>MTKIALIGSGQIGAIVGELCLLENLGDLILYDVVPGIPQGKALDLKHFSTILGVNRNILGTNQIEDIKDADIIVITAGVQRKEGMTREDLIGVNGKIMKSVAESVKLHCSKAFVICVSNPLDIMVNVFHKFSNLPHEKICGMAGILDTSRYCSLIADKLKVSAEDVNAVILGGHGDLMVPLQRYTSVNGVPLSEFVKKNMISQNEIQEIIQKTRNMGAEIIKLAKASAAFAPAAAITKMIKSYLYNENNLFTCAVYLNGHYNCSNLFVGSTAKINNKGAHPVEFPLTKEEQDLYTESIASVQSNTQKAFDLIKGHHHHHH[16x]

Malate dehydrogenase (PfMDH, EC 1.1.1.37) is located downstream of PfAspAT in the cytosol of the parasite. It catalyzes the reversible reaction from malate to oxaloacetate using the reduction of NAD+ to NADH, thus aiding in the maintenance of the correct redox environment, crucial for the parasite’s survival particularly during the blood stages. PfMDH is also involved in the shuttle mechanism of the TCA cycle intermediates (malate/oxaloacetate), necessary for electron transfer from cytosolic NADH to the mitochondrial electron transport chain, a validated antimalarial drug target. PfMDH is a globular tetrameric protein, where each monomer is comprised of 326 residues, which form 9 alpha helixes and 11 beta-sheets.

PfMDH-WT crystals belonged to P1 space group and diffracted to 2.4 Å. Molecular replacement yielded a clear solution of 4 tetramers in the asymmetric unit with R/Rfree of 0,25/0,26, respectively. Similarly to other NAD-dependent dehydrogenases, the active sites are located in the cleft between two domains: an N-terminal cofactor-binding domain containing a parallel structure of first six beta-sheets (Rossmann-fold) and C-terminal substrate-binding domain. The oligomeric surfaces of PfMDH can be split into two major groups: AB and AC. These surfaces comprise 1852.9 Å2 (AB) and 1372.1 Å2 (AC), respectively. Active sites from subunits A and B mirror each other and are located in close proximity to the AB interface (but well separated from each other and interface residues) and distal to the AC interface. The AB interface is mainly formed by residues that belong to alpha helixes 1, 2, 5 and 8 from both subunits. The loop region between α6 and β8 of each subunit (residues 187–192) was found reaching in the hydrophobic pocket region between β7 and β10 of adjacent subunit, facilitating the AC oligomeric contact. Analysis of the crystal structure of PfMDH showed that AB assembly is highly similar to that of the active E. coli dimer. Significantly reduced specific activity, decreased thermal stability and a shift to a lower oligomeric state observed for PfMDH-V190W and PfMDH-E18W mutants suggest that tetrameric assembly of PfMDH is crucial for its catalytic activity, although the AC and AB interfaces are well separated from the active sites.>MGSSHHHHHHSSGLVPRGSHMSNQNAPTPPPTEVIQLDWWKNCVLYQIYPRSFKDSDGDGIGDLKGIISELKHFVDAGVDAIWMSPIFESPMVDFGYDISNFYDIHYEYGTMEDFEELLDKAHELGLKVLLDFVPNHASNESEYFIKSEAREPGYE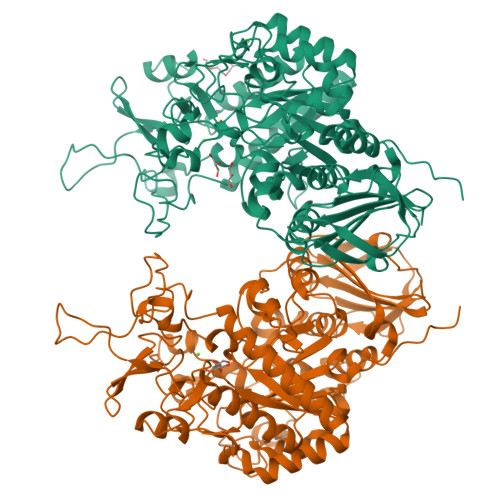NFFIWADPLPNPENPGVRLPPSNWVSQFGGSAWEWSEKRQQYYLHQFAIQQVDFDFRNPAVKQEMFNIMKFWLDKGADGFRLDALPYLIEADPADHEGRYPDDPLSGLTQFESHQLGYTIPLYTKDLIELYDVVYEWREFLDEYNKNHGGDTRVVFSEGYANVSMTMLYYGNEDGAIGAHFPFNFDFITDLSSKSNARDFVYIILRWLTYMPYGGIPNWVFGNHDNNRMPTRFRHDMVDGLNIINMLLPGVAVTYQGEEIGMRDGYVSWEDTVDIEACNRGDPDTYHLYSRDPARTPYHWDNSTSAGFSTSTNTWLPVAEDYQEINLAKQKETARSHFKNYQALTKLRKQATLSHGEYDIRALSDRTFYLVRSLPTHDTYVLLFNVSERRDTVDLGRVPHLTLPATVYVSSIHSARLAGHEITSSQLSLEAGEALVLKAQPI[2x]> DCSSSWSSYEGHCYKAFKQSKTWADAESFCTKQVNGGHLVSIESSGEADFVAHLIAQKIKSAKIHVWIGLRAQNKEKQCSIEWSDGSSISYENWIEEESKKCLGVHKATGFRKWENFYCEQRDPFVCEA;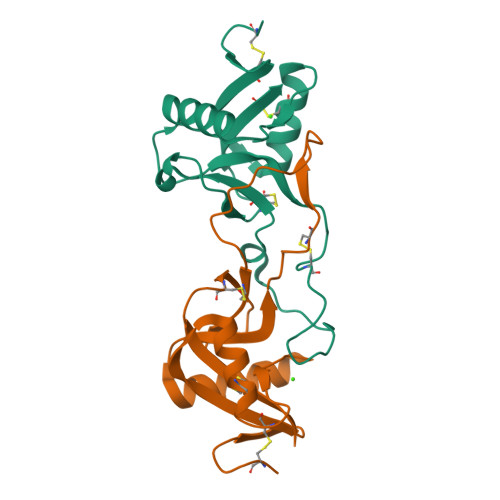> DCPSDWSSYEGHCYKPFNEPKNWADAENFCTQQHTGSHLVSFQSTEEADFVVKLAFQTFDYGIFWMGLSKIWNQCNWQWSNAAMLKYTDWAEESYCVYFKSTNNKWRSITCRMIANFVCEFQA> MSTQYETQGYTINNAGRRLVVDPITRIDGHMRCEVNINDQNVITNAVSCGTMFRGLEIILQGRDPRDAWAFVERICGVCTGVHALASVYAIEDAIGIKVPDNANIIRNIMLATLWCHDHLVHFYQLAGMDWIDVLDALKADPRKTSELAQSLSSWPKSSPGYFFDVQNRLKKFVEGGQLGIFRNGYWGHPQYKLPPEANLMGFAHYLEALDFQREIVKIHAVFGGKNPHPNWIVGGMPCAINIDESGAVGAVNMERLNLVQSIITRTADFINNVMIPDALAIGQFNKPWSEIGTGLSDKCVLSYGAFPDIANDFGEKSLLMPGGAVINGDFNNVLPVDLVDPQQVQEFVDHAWYRYPNDQVGRHPFDGITDPWYNPGDVKGSDTNIQQLNEQERYSWIKAPRWRGNAMEVGPLARTLIAYHKGDAATVESVDRMMSALNLPLSGIQSTLGRI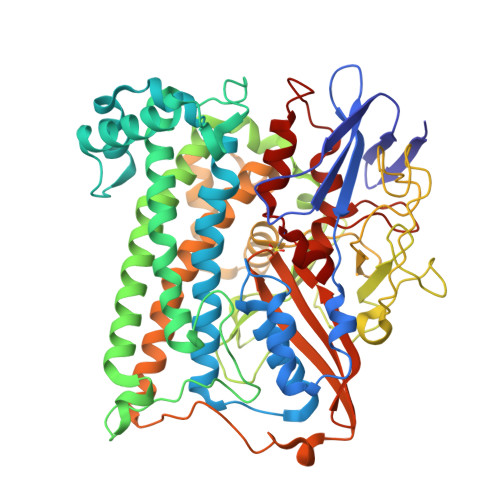LCRAHEAQWAAGKLQYFFDKLMTNLKNGNLATASTEKWEPATWPTECRGVGFTEAPRGALGHWAAIRDGKIDLYQCVVPTTWNASPRDPKGQIGAYEAALMNTKMAIPEQPLEILRTLHSFDPCLACSTH> KLPTNLAYERSIDPSDVCFFVVWPDDRKTPLTYNSRTLLGQMEAKSLAYDVSGQPIKSATAEALAQGNPHQVDFCHVPYGASHIECSFSVSFSSELRQPYKCNSSKVKQTLVQLVELYETKIGWTELATRYLMNICNGKWLWKN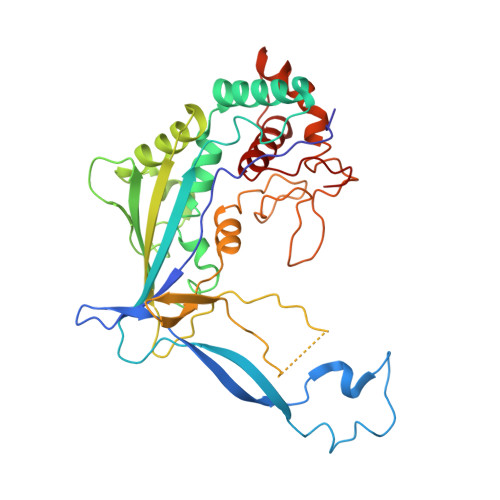TRKAYCWNIVLTPWPWNGEKVGFEDIRTNYTSRQDFKNNKNWSAIVEMIKTAFSSTDGLAIFEVRATLHLPTNAMVRPSQVFTEKEAAAAAAATQNSRVFQSTTIDGERSPILGAFKTGAAIATIDDWYPEATEPLRVGRFGVHREDVTCYRHPSTGKDFFSILQQAEHYIEVLSANKTPAQETINDMHFLMANLIKGGMFQHKGD>[4x]MAHHHHHHVDDDDKMQDRMYQRFLRQHVD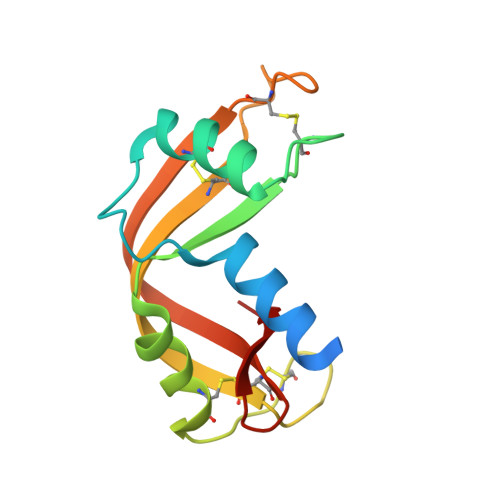PDATGGNDAYCNLMMQRRKMTSHYCKRFNTFIHEDIWNIRSICSTSNIQCKNGQMNCHEGVVKVTACRETGSSRAPNCRYRAMASTRRVVIACEGNPEVPVHFDK> GSSHHHHHHSSGRENLYFQGQAPSFKAEAVFGDNTFGEVSLSDFIGKKYVLLYFYPLDFTFVCPSEIIALDKALDSFKERNVELLGCSVDSKFTHLAWKKTPLSQGGIGNIKHTLISDISKSIARSYDVLFNESVALRAFVLIDKQGVVQHLLVNNLALGRSVDE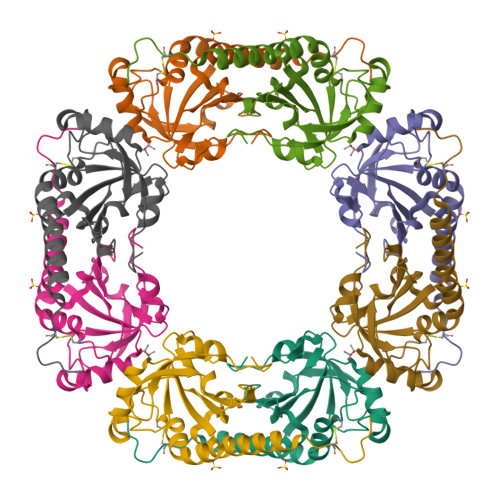ILRLIDALQHHEKYGDVCPANWQKGKESMKPSEEGVAKYLSNL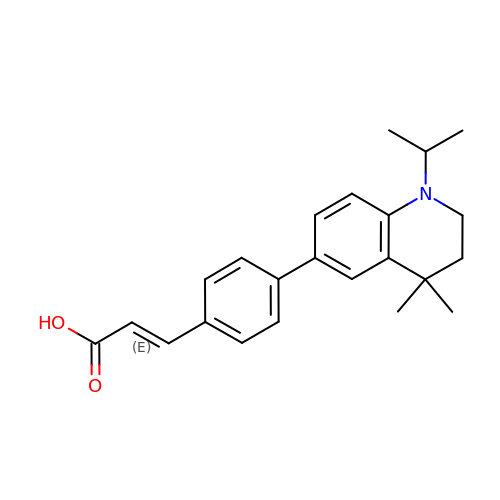(~{E})-3-[4-(4,4-dimethyl-1-propan-2-yl-2,3-dihydroquinolin-6-yl)phenyl]prop-2-enoic acid | C23 H27 N O2 | CBXGBVMKROHWAL-KPKJPENVSA-N>HHHHHHSSGLVPRGSHMLIDTHVHLNDEQYDD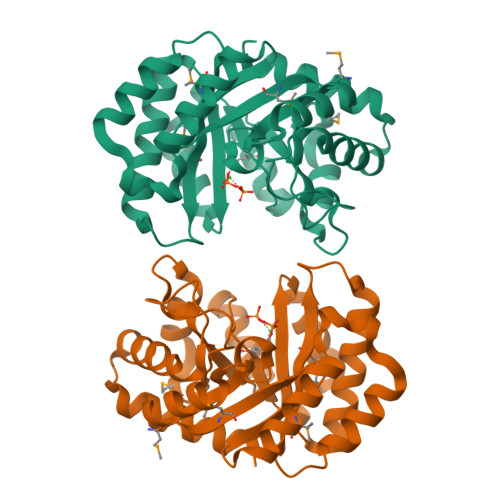DLSEVITRAREAGVDRMFVVGFNKSTIERAMKLIDEYDFLYGIIGWHPVDAIDFTEEHLEWIESLAQHPKVIGIGEMGLDYHWDKSPADVQKEVFRKQIALAKRLKLPIIIHNREATQDCIDILLEEHAEEVGGIMHSFSGSPEIADIVTNKLNFYISLGGPVTFKNAKQPKEVAKHVSMERLLVETDAPYLSPHPYRGKRNEPARVTLVAEQIAELKGLSYEEVCEQTTKNAEKLFNLNS[2x]> 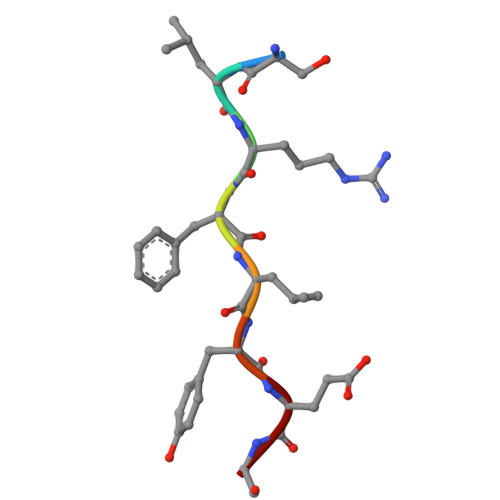SLRFLYEG5-(trifluoromethyloxy)-1,3-dihydroindol-2-one 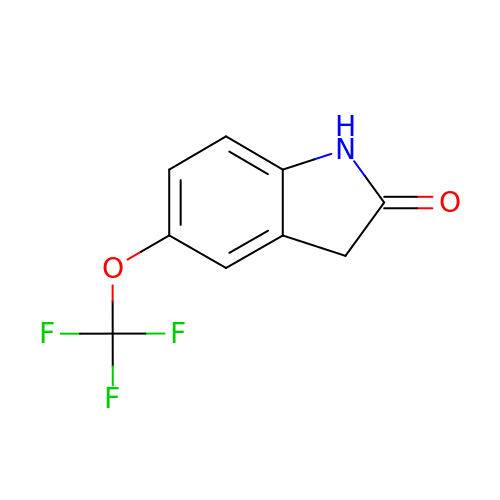| C9 H6 F3 N O2 | NJZFZLIOCDIELL-UHFFFAOYSA-N> MGSSHHHHHHENLYFQGHSSGKDLNISLPLKTKSIAPYETDVPVKIGAAESLFKTNDQGKIEKALVKSYHQPNDTTLDIELKDNIKFQNGQKLTAEKVKSSLENSMKKSDLVKYSLPISSITAKGQKLTIKTNSAYPELVSELANPFMAIYDTDAKSDVNQTPVGTGPYQIKDYKQSRKISLSNFKDYWQGKPKLDHITVTYQEDGNNRVRNLESQKDDLITDVPVNKVQDIENNQNLKVSKESGFRTSLLMYN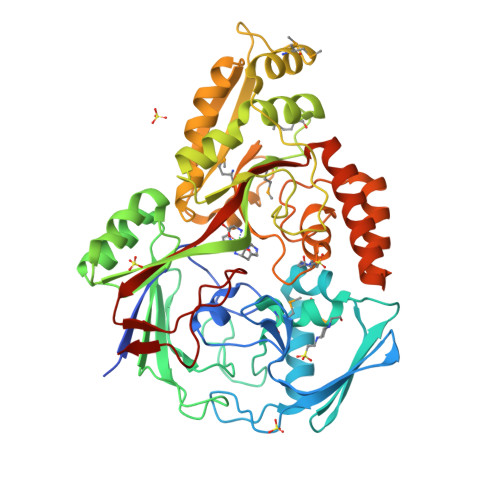HTNKKMTKSVREALDHIIDRQGIADHIYQGYAKPATSPFNDKIPYIKEPKLTKQNIEQAKMLLAKDGYTKEHPLKIKLITYDGRPELSKIAQVLQSDAKKANIEIDIKSVDDIEGYLKDRSAWDATMYSFGTIPRGDTGYFFNQAYKKDGAINKGDYNNSNVDDLINQLNHTVDVKERHNISNDIIKLSSRDVPNSYIAYNDQIVAANSKVKNYKVTPEGIYLIDYRTTIER>[5x]APAANPAVTESVAPTTAPAPAAAAPESITPVNPAPTIQPPETRGMDLSIWGMYQHADAVVKAVMIGLVLASIVT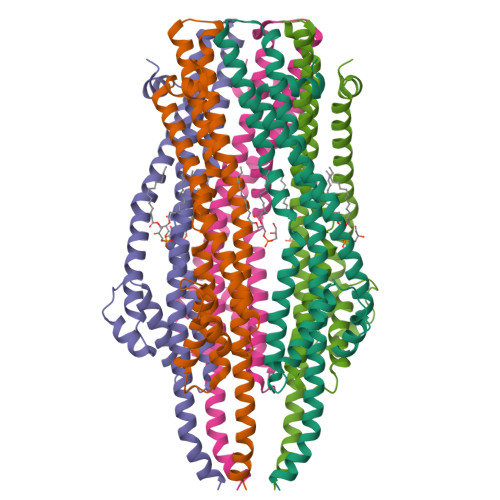WTILFAKGSELLRAKRRLRREQLALAEARSLDEASELAQNFSPESVSAVLLNDAQNELELSAESNDNNGIKERTGFRLERRVAAYSRNMGRGNGFLATIGAISPFVGLFGTVWGIMNSFIGIAHSQTTNLAVVAPGIAEALLATAMGLVAAIPAVVIYNIFARVISGHRAQVGDVAAQVLLLQGRDLDLAATAEAKRSQHAHQLRAGHHHHHH>MTRRILVTGSSRGIGKAIALQLAKAGFDVTVHARSRQAEAEQVVQEIQALGQNSHYLMFDVNERQTVQQILEQDVEQHGGFYGVVLNAGLTHDGAFPALTDQDWDEVISTSLDGFYNVLKPLIMPMIHLRKGGRIVTLSSVSGIMGNRGQVNYSAAKAGLIGATKALALELAKRKITV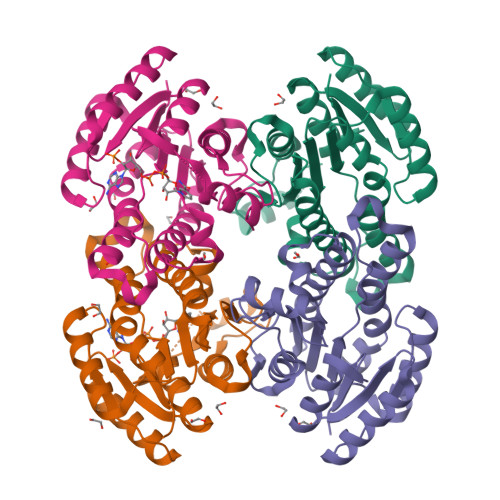NCVAPGLIETEMVTDEVKEHALKMIPLQRMGQVDEVASVVKFLCSDEASYVTRQVISVNGGLI[4x]3-[[1-(cyclopropylmethyl)-5-ethanoyl-6,7-dihydro-4~{H}-pyrazolo[4,3-c]pyridin-3-yl]amino]-~{N}-propan-2-yl-benzamide 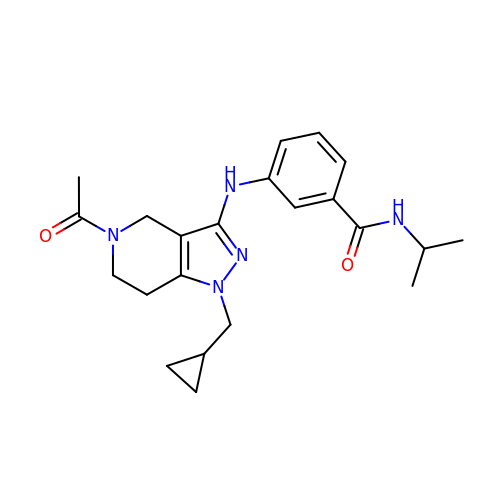| C22 H29 N5 O2 | KDQSAWDSOXZXES-UHFFFAOYSA-N(2R)-2-[[3-[[4-[(Z)-(4-OXO-2-SULFANYLIDENE-1,3-THIAZOLIDIN-5-YLIDENE)METHYL]PHENYL]METHYLAMINO]PHENYL]CARBONYLAMINO]PENTANEDIOIC 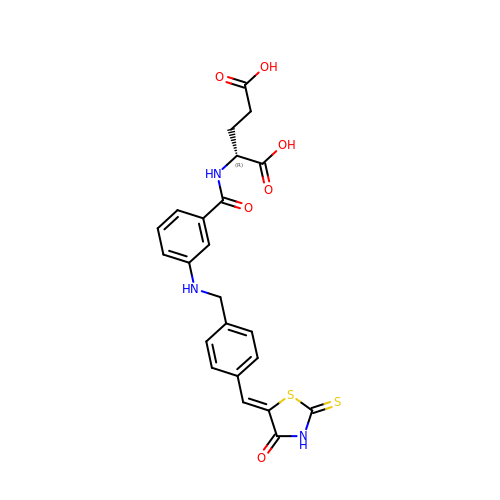ACID | C23 H21 N3 O6 S2 | ZDOPULPHJIBVJX-RMFUMNGISA-N> MTKTAFLFAGQGAQYLG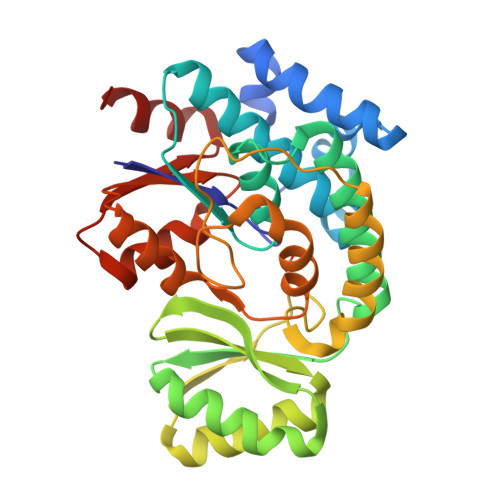MGRDFYDQYPIVKETIDRASQVLGYDLRYLIDTEEDKLNQTRYTQPAILATSVAIYRLLQEKGYQPDMVAGLSLGEYSALVASGALDFEDAVALVAKRGAYMEEAAPADSGKMVAVLNTPVEVIEEACQKASELGVVTPANYNTPAQIVIAGEVVAVDRAVELLQEAGAKRLIPLKVSGPFHTSLLEPASQKLAETLAQVSFSDFTCPLVGNTEAAVMQKEDIAQLLTRQVKEPVRFYESIGVMQEAGISNFIEIGPGKVLSGFVKKIDQTAHLAHVEDQASLVALLEKL>SNAMKEKVVSLAQDLIRRPSISPNDEGCQQIIAERLEKLGFQIEWMPFNDTLNLWAKHGTSEPVIAFAGHTDVVPTGDENQWSSPPFSAEIIDGMLYGRGAADMKGSLAAMIVAAEEYVKANPNHKGTIALLITSDEEATAKDGTIHVVETLMARDEKITYCMVGEPSSAKNLGDVVKNGRRGGGFLTKPGKLLDSITSAIEETIGITPKAETGGGTSDGRFIALMGAEVVEFGPLNSTIHKVNECVSVEDLGKCGEIYHKMLVNLLDS[2x]

DapE hydrolyzes N-succinyl-L,L-diaminopimelic acid to L,L-diaminopimelic acid and succinate, is part of a biosynthetic pathway that is the major source of lysine in bacteria, and is essential for cell growth and proliferation. All the DapE enzymes characterized to date belong to the M20 family of dinuclear Zn(II)-dependent metalloproteases. In order to examine the role of the catalytic domain of DapE enzymes and the role of the active site loops, we have engineered the HiDapE and the DapE from Vibrio cholerae (VcDapE) by deleting their dimerization domains. Removal of the dimerization domain in DapE enzymes renders the enzyme inactive, even though the resulting truncated proteins have structures of the catalytic domain that are remarkably similar to WT-DapE and AAP.

Deletion of the dimerization domain led to a monomeric structure for HiDapET. The monomeric nature of HiDapET in solution was corroborated by size exclusion chromatography (SEC) and dynamic light scattering (DLS). The structure of HiDapET was determined and refined at 1.84 Å resolution and the final model shows two independent monomers in the asymmetric unit. Two zinc atoms were found in the active site and reside in the same position as in dimeric structure of WT-HiDapE separated by 3.40 Å. Superimposition of the active site regions shows nearly identical conformations of main chain and side chains with rmsd as low as 0.15 Å for the metal ions and side chains of residues involved in their coordination. Larger differences within the active site area are observed in two regions containing solvent exposed loops. Region I (residues 176–187) has been engineered to replace what was originally the connector/hinge region formed by two loops linking the catalytic domain with the dimerizaton domain (Region I). This region is highly flexible and is disordered in the crystal structure of HiDapET (no electron density observed for residues 182–187). Region II (residues 209–224), which corresponds to a loop overhanging the active site metal ions (loop V, vide infra) adopts a different conformation in comparison to that observed in the HiDapE structure (rmsd of 1.5 Å between the structures). The structure of [ZnZn(HiDapET)] is virtually identical to the catalytic domain the WT-HiDapE with an rmsd of 0.8 Å for 248 equivalent Cα atoms.> MRIEDKLYLNRYR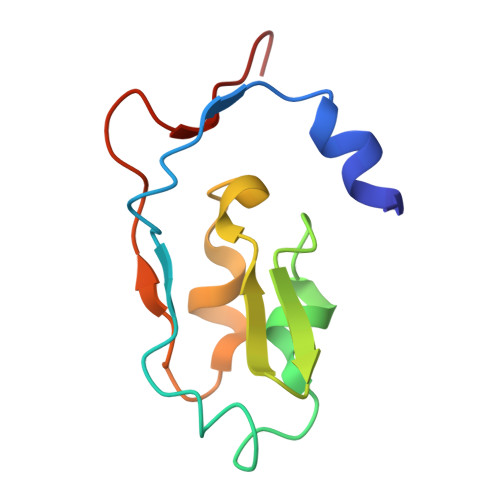TDEENPHLKIKDESICAEKCSDRPCVSCCPADVYEWTESGMEVKFEGCLECGTCRIVCPFGNIEWNYPRGNYGVLYKFG>[3x]PIQVIEDDRNNRGTEPFVTGVRGQVPPLVTTNFLVKDQGNASPRYIRCTSYNIPCTSDMAKQAQVPLAAVIKPLARLPPEE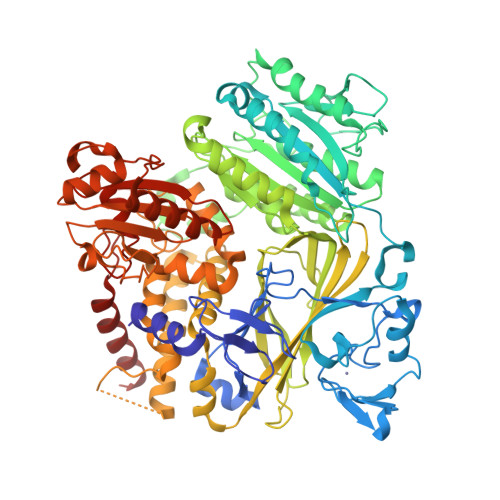ASPYVVDHGESGPLRCNRCKAYMCPFMQFIEGGRRFQCCFCSCINDVPPQYFQHLDHTGKRVDAYDRPELSLGSYEFLATVDYCKNNKFPSPPAFIFMIDVSYNAIRTGLVRLLCEELKSLLDFLPREGGAEESAIRVGFVTYNKVLHFYNVKSSLAQPQMMVVSDVADMFVPLLDGFLVNVNESRAVITSLLDQIPEMFADTRETETVFVPVIQAGMEALKAAECAGKLFLFHTSLPIAEAPGKLKNRDDRKLINTDKEKTLFQPQTGAYQTLAKECVAQGCCVDLFLFPNQYVDVATLSVVPQLTGGSVYKYASFQVENDQERFLSDLRRDVQKVVGFDAVMRVRTSTGIRAVDFFGAFYMSNTTDVELAGLDGDKTVTVEFKHDDRLNEESGALLQCALLYTSCAGQRRLRIHNLALNCCTQLADLYRNCETDTLINYMAKFAYRGVLNSPVKAVRDTLITQCAQILACYRKNCASPSSAGQLILPECMKLLPVYLNCVLKSDVLQPGAEVTTDDRAYVRQLVTSMDVTETNVFFYPRLLPLTKSPVESTTEPPAVRASEERLSNGDIYLLENGLNLFLWVGASVQQGVVQSLFSVSSFSQITSGLSVLPVLDNPLSKKVRGLIDSLRAQRSRYMKLTVVKQEDKMEMLFKHFLVEDKSLSGGASYVDFLCHMHKEIRQLLS> HHHHHHNRPRFT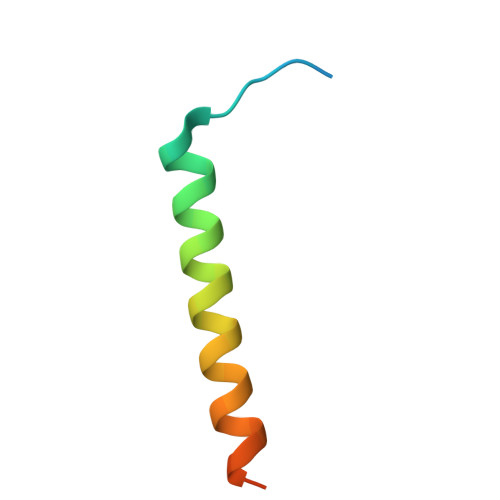LQELRDVLQERNKLKSQLLVVQEELQCYKSG>GAMASARSLRSLQRQRAILKVMNTIGGVAYLREQFYESVSKYMGSTTTLDKKTVRGDVDLMVESEKLGARTEPVSGRKIIFLPTVGEDAIQRYILKEKDS[2x]

Recruitment of Pol III to these genes requires the essential transcription factors TFIIIB and TFIIIC2. The six subunits of yeast TFIIIC are partitioned into two DNA-binding subcomplexes (τA and τB). The binding of these intragenic promoters by TFIIIC permits the assembly of TFIIIB, upstream of the transcription start site, which subsequently leads to the recruitment of Pol III, the formation of a PIC and finally to transcription. A genetic study suggests that the two largest TFIIIC subunits, τ138 and τ131, are responsible for connecting τA and τB16.

The τ138 subunit is currently the least well-characterized subunit of TFIIIC. We first solved the structure of the central domain of τ138 (546–641) using the sulphur-SAD technique. The 1.4 Å crystal structure (Rwork/Rfree of 17.5%/19.8%) of this domain reveals a canonical winged helix domain that contains an additional C-terminal helix. This first structurally characterized part of τ138 thus represents an ‘extended' winged helix (eWH) domain35. The eWH domain is moderately well conserved from yeast to human, and contains basic patches that could also suggest a role in binding nucleic acids. However, we only detect very weak unspecific binding of the eWH domain to single and double-stranded DNA. Isothermal titration calorimetry (ITC) did not detect an interaction between the eWH and the TPR array. However, when we tested a construct that contained the eWH domain with additional residues at the C terminus (546–693), we observed a Kd for the interaction with the TPR array of ∼100 nM. We thus concluded that the region 641–693 of τ138, hereafter referred to as ‘τ131-Interaction Region (τIR)', is necessary and sufficient to bind the TPR array of τ131. Interestingly, the removal of just the eWH domain is also lethal to yeast, indicating that despite it being dispensable for the interaction with τ131 in vitro, it is still essential for proper TFIIIC function in vivo.ethyl 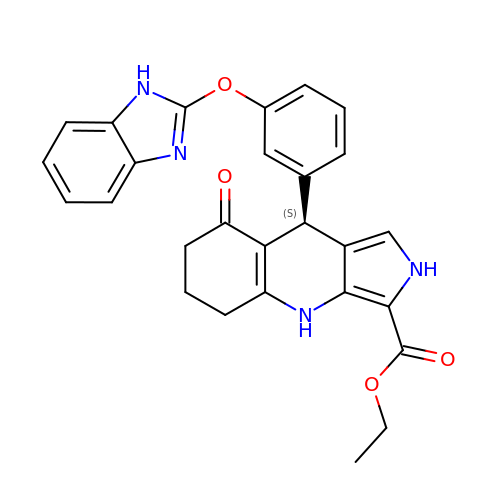(9S)-9-[3-(1H-benzimidazol-2-yloxy)phenyl]-8-oxo-4,5,6,7,8,9-hexahydro-2H-pyrrolo[3,4-b]quinoline-3-carboxylate | C27 H24 N4 O4 | YXMQIWJYPNBZJS-QFIPXVFZSA-N>[2x]PPYTVVYFPVRGRCAALRMLLADQGQSWKEEVVTVETWQEGSLKASSLYGQLPKFQDGDLTLYQSNTILRHLGRTLGLYGKDQQEAALVDMVNDGVEDLRCKYIS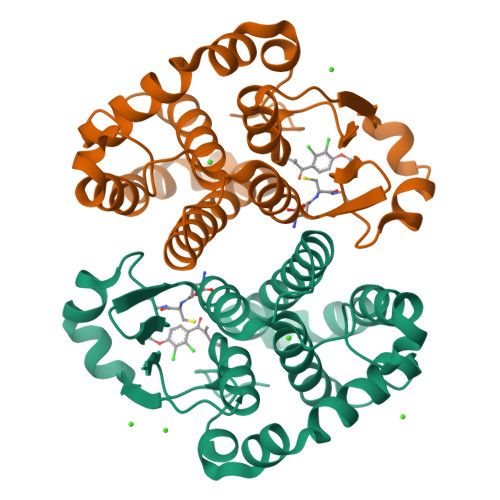LIVTNYEAGKDDYVKALPGQLKPFETLLSQNQGGKTFIVGDQISFADYNLLDLLLIHEVLAPGCLDAFPLLSAYVGRLSARPKLKAFLASPEYVNLPINGNGKQ>[2x]MMIITTMQDAIGRTPVFKFTNKDYPIPLNSAIYAKLEHLNPGGSVKDRLGQYLIGEGFKTGKITSKTTIIEPTAGNTGIALALVAIKHHLKTIFVVPEKFSTEKQQIMRALGALVINTPTSEGISGAIKKSKELAESIPDSYLPLQFENPDNPAAYYHTLAPEIVQELGTNLTSFVAGIGSGGTFAGTARYLKERIPAIRLIGVEPEGSILNGGEPGPHEIEGI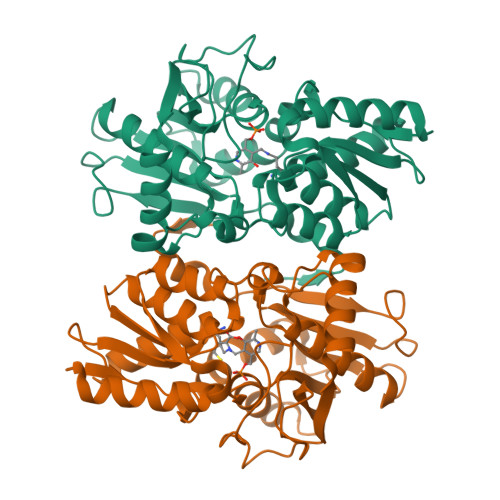GVEFIPPFFENLDIDGFETISDEEGFSYTRKLAKKNGLLVGSSSGAAFVAALKEAQRLPEGSQVLTIFPDVADRYLSKGIYLLQHHHHHH> IP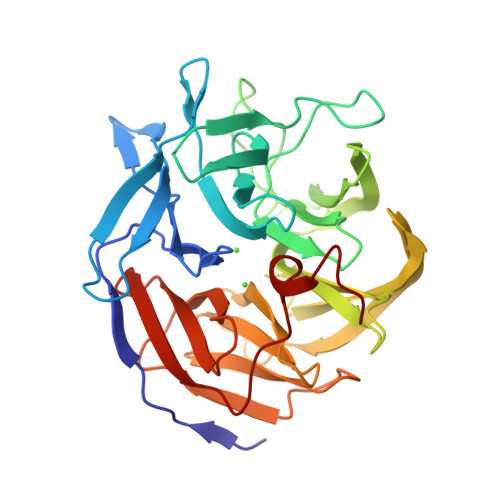VIEPLFTKVTEDIPGAEGPVFDKNGDFYIVAPQVEVNGKPAGEILRIDLKTGKKTVICKPEVNGYGGIPAGCQCDRDANQLFVADMRLGLLVVQTDGTFEEIAKKDSEGRRMQGCNDCAFDYEGNLWITAPAGEVAPADYTRSMQEKFGSIYCFTTDGQMIQVDTAFQFPNGIAVRHMNDGRPYQLIVAETPTKKLWSYDIKGPAKIENKKVWGHIPGTHEGGADGMDFDEDNNLLVANWGSSHIEVFGPDGGQPKMRIRCPFEKPSNLHFKPQTKTIFVTEHENNAVWKFEWQRNGKKQYCETLKFGIF>MFDFDGYMLRKAKSVNKALEAAVQMKEPLKIHESMRYSLLAGGKRVRPMLCIAACELVGGDESTAMPAACAVEMIHTMSLMHDDLPCMDNDDLRRGKPTNHMAFGESVAVLAGDALLSFAFEHVAAATKGAPPERIVRVLGELAVSIGSEGLVAGQVVDVCSEGMAEVGLDHLEFIHHHKTAALLQGSVVLGAILGGGKEEEVAKLRKFANCIGLLFQVVDDILDVTKSSKELGKTAGKDLVADKTTYPKLIGVEKSKEFADRLNREAQEQLLHFHPHRAAPLIALANYIAYRDN[2x];>MQPYWAAIEADIERYLKKSITIRPPETVFGPMHHLTFAAPATAASTLCLAACELVGGDRSQAMAAAAAIHLVHAAAYVHEHLPLTDGSRPVSKPAIQHKYGPNVELLTGDGIVPFGFELLAGSVDPARTDDPDRILRV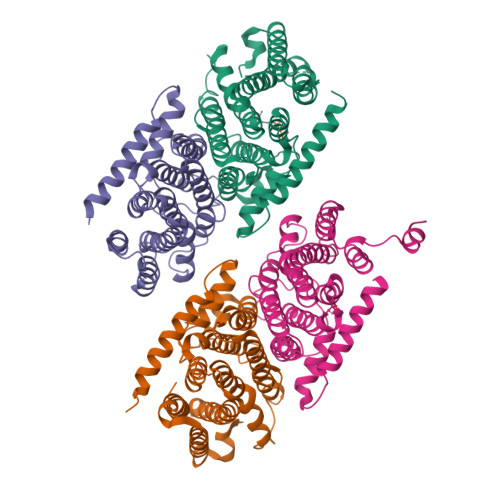IIEISRAGGPEGMISGLHREEEIVDGNTSLDFIEYVCKKKYGEMHACGAACGAILGGAAEEEIQKLRNFGLYQGTLRGMMEMKNSHQLIDENIIGKLKELALEELGGFHGKNAELMSSLVAEPSLYAAHHHHHHHH[2x]> DTVGRPLPHLAAAMQASGEAVYCDDIPRYENELFLRLVTSTRAHAKIKSIDVSEAQKVPGFVCFLSADDIPGSNETGLFNDETVFAKDTVTCVGHIIGAVVADTPEHAERAAHVVKVTYEDLPAIITIEDAIKNNSFYGSELKIEKGDLKKGFSEADNVVSGELYIGGQDHFYLETHCTIAIPKGEEGEMELFVSTQNAMKTQSFVAKMLGVPVNRILVRVKRMGGGFGGKETRSTLVSVAVALAAYKTGHPVRCMLDRNEDMLITGGRHPFLARYKVGFMKTGTIVALEVDHYSNAGNSRDLSHSIMERALFHMDNCYKIPNIRGTGRLCKTNLSSNTAFRGFGGPQALFIAENWMSEVAVTCGLPAEEVRWKNMYKEGDLTHFNQRLEGFSVPRCWDECLKSSQYYARKSEVDKFNKENCWKKRGLCIIPTKFGISFTVPFLNQAGALIHVYTDGSVLVSHGGTEM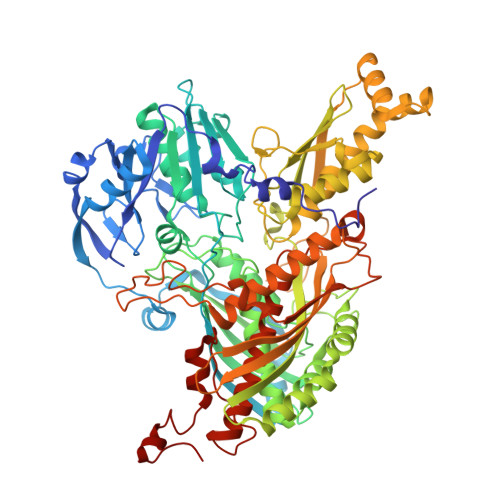GQGLHTKMVQVASKALKIPISKIYISETSTNTVPNSSPTAASVSTDIYGQAVYEACQTILKRLEPFKKKNPDGSWEDWVMAAYQDRVSLSTTGFYRTPNLGYSFETNSGNAFHYFTYGVACSEVEIDCLTGDHKNLRTDIVMDVGSSLNPAIDIGQVEGAFVQGLGLFTLEELHYSPEGSLHTRGPSTYKIPAFGSIPTEFRVSLLRDCPNKKAIYASKAVGEPPLFLGASVFFAIKDAIRAARAQHTNNNTKELFRLDSPATPEKIRNACVDKFTTLCVTGAPGNCK>[2x]SMPAYACQRPSPLTHHNTLLSEALETLAEAAGFEANEGRLLSFSRAASVLKSLPCPVASLSQLHGLPYFGEHSTRVIQELLEHGTCEEVKQVRCSERYQTMKLFTQVFGVGVKTANRWYQEGLRTLDELREQPQRLTQQQKAGLQYYQDLSTPVRRADAEALQQLIEAAVRQTLPGATVTLTGGFRRGKLQGH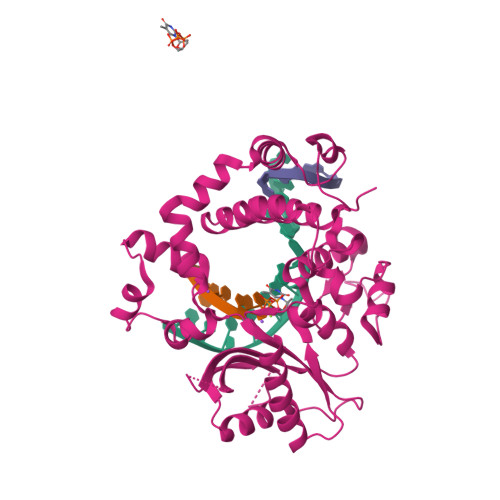DVDFLITHPEEGQEVGLLPKVMSCLQSQGLVLYHQYHRSHLADSAHNLRQRSSTMDVFERSFCILGLPQPQQAALAGALPPCPTWKAVRVDLVVTPSSQFPFALLGWTGSQFFERELRRFSRQEKGLWLNSHGLFDPEQKRVFHATSEEDVFRLLGLKYLPPEQRNA> AKPCTVSTTNATVDLGDLYSFSLMSAGAASAWHDVALELTNCPVGTSRVTASFSGAADSTGYYKNQGTAQN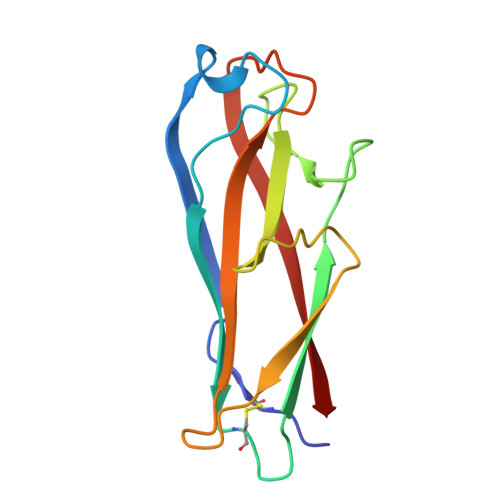IQLELQDDSGNTLNTGATKTVQVDDSSQSAHFPLQVRALTVNGGATQGTIQAVISITYTYS>[2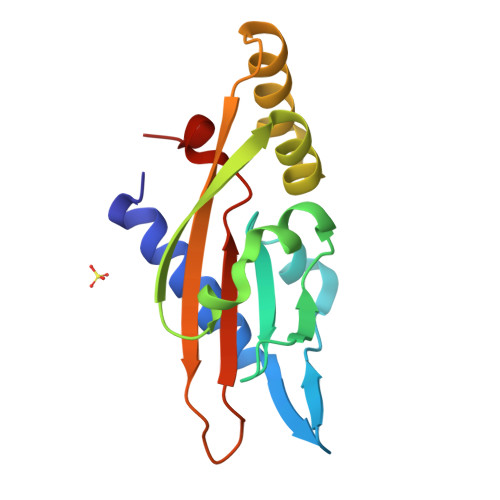x]SFDKTTFRLLRGESNLFYTLAKWENNKLHVELPENIDKQSPTMTLIYDENGQLLWAQRDVPWLMKMIQPDWLKSNGFHEIEADVNDTSLLLSGDHSIQQQLQEVRQNNNNAQMTHSVAVNVYPATSRMPKLTIVVVDTIPVELKSSYM5-(2,5-dioxo-2,5-dihydro-1H-pyrrol-1-yl)-2-(6-hydroxy-3-oxo-3H-xanthen-9-yl)benzoic 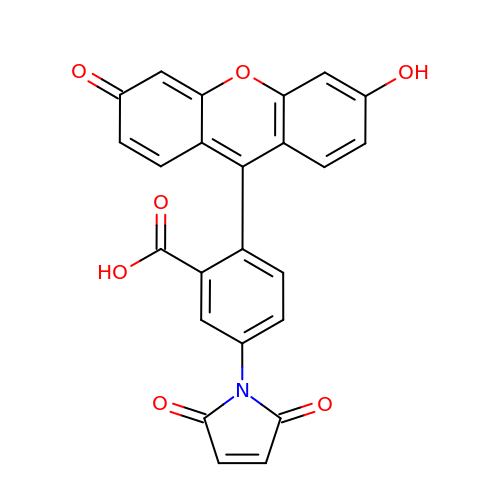acid | C24 H13 N O7 | HFBMFFXWMZRDIY-UHFFFAOYSA-N> MPREIITLQLGQCGNQIGFEFWKQLCAEHGISPEAIVEEFATEGTDRKDVFFYQADDEHYIPRAVLLDLEPRVIHSILNSPYAKLYNPENIYLSEHGGGAGNNWASGFSQGEKIHEDIFDIIDREADGSDSLEGFVLCHSIAGGTGSGL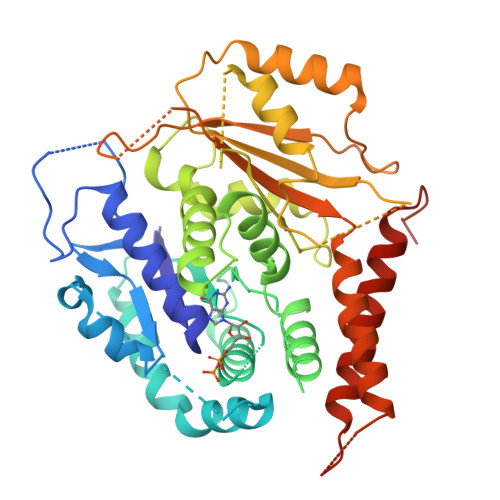GSYLLERLNDRYPKKLVQTYSVFPNQDEMSDVVVQPYNSLLTLKRLTQNADCLVVLDNTALNRIATDRLHIQNPSFSQINQLVSTIMSASTTTLRYPGYMNNDLIGLIASLIPTPRLHFLMTGYTPLTTDQSVASVRKTTVLDVMRRLLQPKNVMVSTGRDRQTNHCYIAILNIIQGEVDPTQVHKSLQRIRERKLANFIPWGPASIQVALSRKSPYLPSAHRVSGLMMANHTSISSLFERTCRQYDKLRKREAFLEQFRKEDMFKDNFDEMDTSREIVQQLIDEYHAATRPDYISWGTQEQ>[2x]SAQQYQGIYVWRVENFSHHLRNQEAGQPIVLHSPPFYTGRPGYKLCLRLHLQTPSAPRCSNFISLFVHTMQGEFDSQLSWPLQGTIRLAVLDQVEGQHHIEVMETKPDLQAFQRPTVMRNPK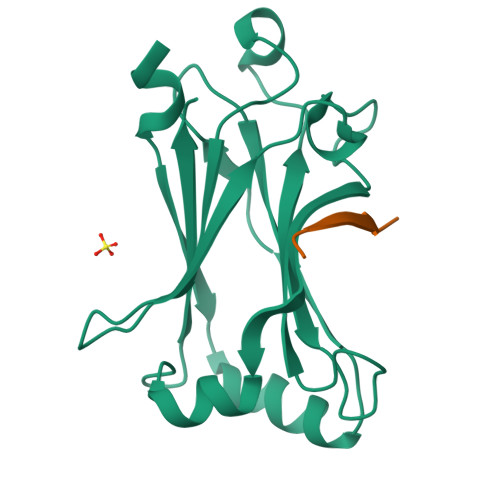GFGYVTFLHLQALRQRGFVKEDVLLVRCEVTPRFD;>EPVETTDY[2x]> KSCPNPGAIANGQIDVPGGILFGATISFSCNTGYKLAGSTSSFCLISGSSVQWSDPLPECREIY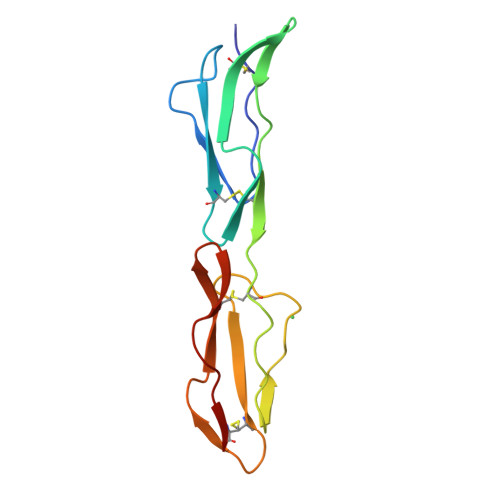CPAPPQIDNGIIQGERDHYGYRQSVTYACNKGFTMIGEHSIYCTVNNDAGEWSGPPPECRG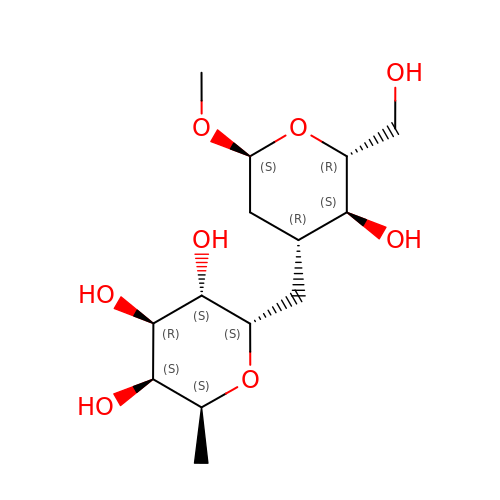(2~{S},3~{S},4~{R},5~{S},6~{S})-2-[[(2~{R},3~{S},4~{R},6~{S})-2-(hydroxymethyl)-6-methoxy-3-oxidanyl-oxan-4-yl]methyl]-6-methyl-oxane-3,4,5-triol | C14 H26 O8 | ZKQNJYZBKMAROQ-UDZHPATASA-N>[2x]GTGSRPITDVVFVGAARTPIGSFRSAFNNVPVTVLGREALKGALKNANVKPSLVQEAFIGVVVPSNAGQGPARQVVLGAGCDVSTVVTAVNKMSASGMKAIACAASILQLDLQEMVVAGGMESMSCVPFYLPRGEIPFGGTKLIDGIPRDGLNDVYNDILMGACADKVAKQFAITREEQDKYAILSYKRSAAAWKEGIFAKEIIPLEVTQGKKTITVEEDEEYKKVNFEKIPK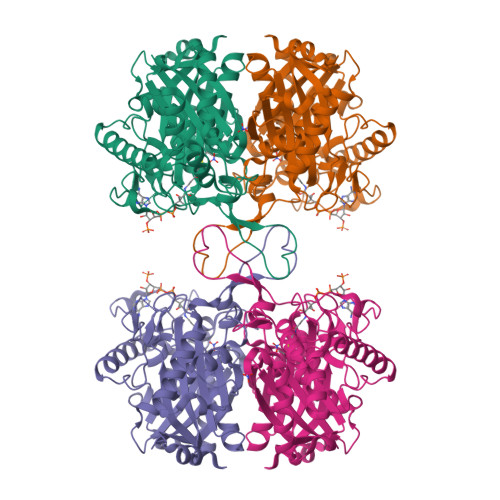LKPAFTSEGSVTAANASTLNDGAAMVVMTTVDGAKKHGLKPLARMLAYGDAATHPIDFGIAPASVIPKVLKLAGLQIKDIDLWEINEAFAVVPLYTMKTLGLDESKVNIHGGAVSLGHPIGMSGARIVGHLVHTLKPGQKGCAAICNGGGGAGGMIIEKL>[4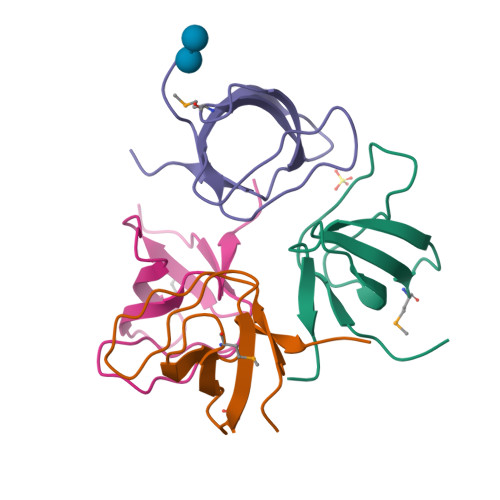x]GSEQTHRAIFRFVPRHEDELELEVDDPLLVELQAEDYWYEAYNMRTGARGVFPAYYAIEVTK>[6x]DYGRADNENRVGQVTGLAWTEVGGDLLTIETACVPGKGKLTYTGSLGEVMQESIQAALTVVRARAEKLGINPDFYEKRDIHVHVPEGATPKDGPAA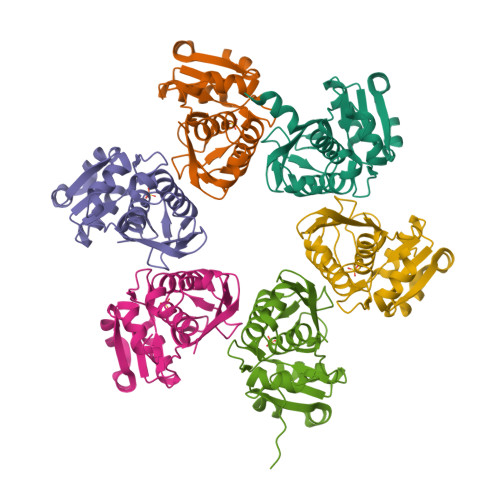GIAMCTALVSCLTGNPVRADVAMTGEITLRGQVLPIGGLKEKLLAAHRGGIKTVLIPFENKRDLEEIPDNVIADLDIHPVKRIEEVLTLALQNEPSGMQVVTAK> MKADNPFDLLLPAAMAKVAEEAGVYKATKHPLKTFYLAITAGVFISIAFVFYITATTGTGTMPFGMAKLVGGICFSLGLILCVVCGADLFTSTVLIVVAKASGRITWGQLAKNWLNVYFGNLVGALLFVLLMWLSGEYMTANGQWGLNVLQTADHKVHHTFIEAVCLGILANLMVCLAVWMSYSGRSLMDKAFIMVLPVAMFVASGFEHSIANMFMIPMGIVIRDFASPEFWTAVGSAPENFSHLTVMNFITDNLIPVTIGNIIGGGLLVGLTYWVIYLRENDHH

FocA belongs to the widespread, evolutionarily ancient formate-nitrite transporter (FNT) family of pentameric anion channels and translocates formic acid bidirectionally. Central to the FNT family’s function are conserved histidine and threonine residues (H209 and T91 in E. coli FocA), both of which are essential for pH-dependent formate:H+ symport into fermenting E. coli cells. Here, we show the high-resolution structure of native E. coli FocA, together with the H209N variant, and describe the dynamic pore features that couple to the protonation state.

Here, we identify compartmentalized polarity distribution across the complete FocA pore structure – resolved at 2.56 Å – mirrored against a two-fold axis with H209 at its center. Thereafter, 3665 micrographs were collected, displaying clear side and top views of the pentameric protein complex, leading to high-quality 2D class averages. The final FocA structure was reconstructed from 302,937 single-particles, achieving a resolution of 2.56 Å (FSC = 0.143), and showing a thorough sampling across orientations (Sampling Compensation Factor (SCF) = 0.87, Supplementary Fig. 3H), with the local resolutions being ~2.3-2.7 Å. In addition, compared to HSC’s pore-forming N-terminus and PfFNT’s β-barrel, FocA’s N-terminus forms a loop parallel to the pentameric cytoplasmic face, creating the flattest surface among known FocA structures, and generally among FNTs. This flatness of the surface is imposed by the entirely flat positioning of the N-terminal α-helix on the cytosolic face of the FocA pentamer, as compared to other FNTs. Resolving the complete FocA structure allows us to trace the formate channel in the native assembly. The channel is constrained by mainly hydrophobic residues, especially phenylalanine, whereas the periplasmic side displays a partially positive charge, conveyed by lysine (K68 and K165) and histidine (H155) residues. The formate channel around this key residue is highly constrained: while the H209 is coordinated by an interaction with T91 (dvdw = 3.6 Å), which supports in vivo data indicating that this represents the open channel, the channel’s path itself is sterically confined by two opposing phenylalanine residues (F75 and F202), forming a spatial gate. In addition, side chain flexibility can modulate the effective pore diameter, as illustrated by comparing the “radius”, defined by the side chain atoms, with the “free radius”, based on the main chain atoms. The difference between these radii suggests that side chain flexibility can act both as a steric barrier that shifts dynamically and as a mechanism of substrate selectivity, since the substrate must remain in contact with the side chains to pass. In particular, the Phe-gate of F75 and F202 plays a crucial role in this dynamic channel range.>GTTKHSKLLILGSGPAGYTAAVYAARANLQPVLITGMEKGGQLTTTTEVENWPGDPNDLTGPLLMERMHEHATKFETEIIFDHINKVDLQNRPFRLNGDNGEYTCDALIIATGASARYLGLPSEEAFKGRGVSASATCDGFFYRNQKVAVIGGGNTAVEEALYLSNIASEVHLIHRRDGFRAEKILIKRLMDKVENGNIILHTNRTLEEVTGDQMGVTGVRLRDTQNSDNIESLDVAGLFVAIGHSPNTAIFEGQLELENGYIKVQ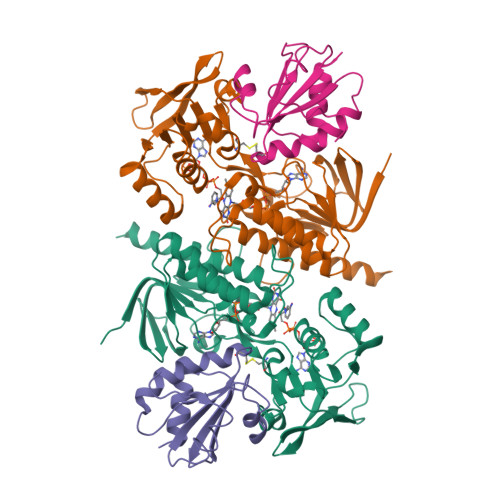SGIHGNATQTSIPGVFAAGDVMDHIYRQAITSAGTGCMAALDAERYLDGLADAK[4x];>[4x]SDKIIHLTDDSFDTDVLKADGAILVDFWAEWCGPSKMIAPILDEIADEYQGKLTVAKLNIDQNPGTAPKYGIRGIPTLLLFKNGEVAATKVGALSKGQLKEFLDANLA> GSMTPTPTILTSGTYNDSLLTINSDYDAYLLDFPLMGDDFMLYLARMELKCRFRRHERVLQSGLCVSGLTINGARNRLKRVQLPEGTQIIVNIGSVDIMRGKPLVQIEHDFRLLIKEMHNMRLVPILTNLAPLGNYCHDKVLCDKIYRFNKFIRSE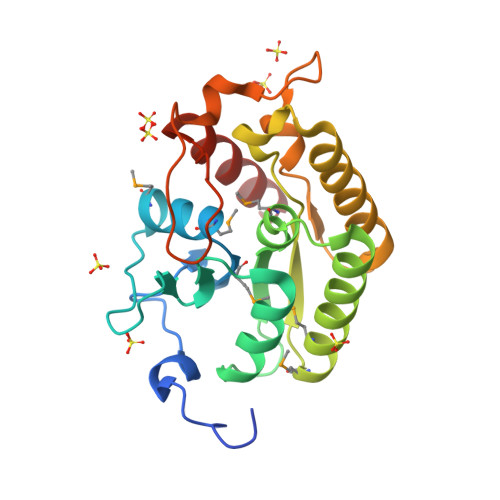CCHLKVIDIHSCLINERGVVRFDCFQASPRQVTGSKEPYLFWNKIGRQRVLQVIETSLEY>MDHHHHHHLPNITILATGGTIAGGGDSATKSNYTVGKVGVENLVNAVPQLKDIANVKGEQVVNIGSQDMNDNVWLTLAKKINTDC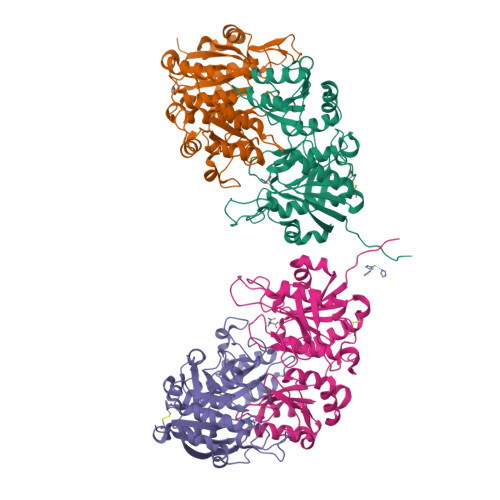DKTDGFVITHGVDTMEETAYFLDLTVKCDKPVVMVGAMRPSTSMSADGPFNLYNAVVTAADKASANRGVLVVMNDTVLDGRDVTTTNTTDVATFKSVNYGPLGYIHNGKIDYQRTPARKHTSDTPFDVSKLNELPKVGIVYNYANASDLPAKALVDAGYDGIVSAGVGNGNLYKSVFDTLATAAKTGTAVVRSSRVPTGATTQDAEVDDAKYGFVASGTLNPQKARVLLQLALTQTKDPQQIQQIFNQY[4x]>MRDMEFIEWYPRGYGVAFKVKRKILEEQSEYQKIEVYETEGFGKLLAIDGTVQLVTEGEKSYHEPLVHPAMLAHPNPRRVLIIGGGDGGAIREVLKHEEVEEVIMVEIDKKVIEISAKYIGIDGGILEKMLSDKHEKGKLIIGDGVKFIEENSGFDVIIVDSTDPVGPAEMLFSEEFYKNAYRALNDPGIYVTQAGSVYLFTDEFLTAYRKMRKV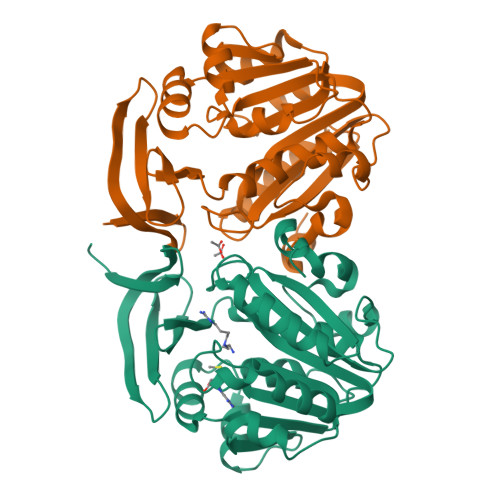FDKVYYYSFPVIGYASPWAFLVGVKGSIDFMKVDAEKGKKLGLEYYDPDKHETLFQMPRYIVQML[4x]>[2x]MTMVGLI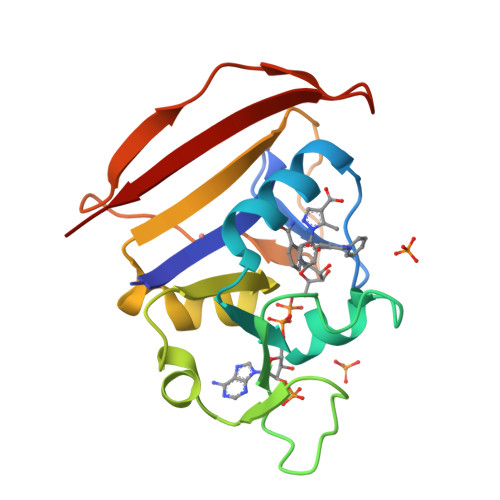WAQATSGVIGRGGDIPWRLPEDQAHFREITMGHTIVMGRRTWDSLPAKVRPLPGRRNVVLSRQADFMASGAEVVGSLEEALTSPETWVIGGGQVYALALPYATRCEVTEVDIGLPREAGDALAPVLDETWRGETGEWRFSRSGLRYRLYSYHRS>[2x]SNDYRVAVFGAGGVGKSSLVLRFVKGTFRESYIPTVEDT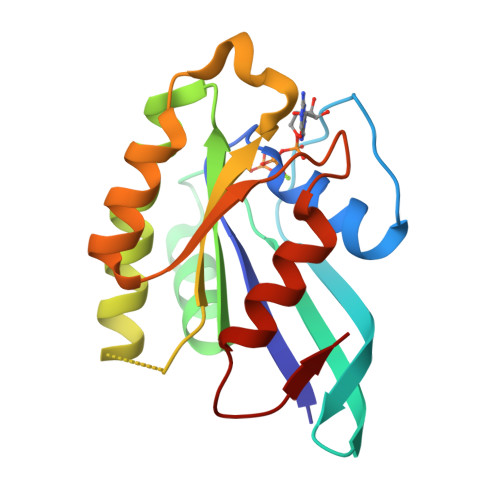YRQVISCDKSICTLQITDTTGSHQFPAMQRLSISKGHAFILVYSITSRQSLEELKPIYEQICEIKGDVESIPIMLVGNKCDESPSREVQSSEAEALARTWKCAFMETSAKLNHNVKELFQELLNLEKRRTVSL N'-[1,1-bis(oxidanylidene)thian-4-yl]-5-ethyl-4-oxidanylidene-7-[3-(trifluoromethyl)phenyl]thieno[3,2-c]pyridine-2-carboximidamide 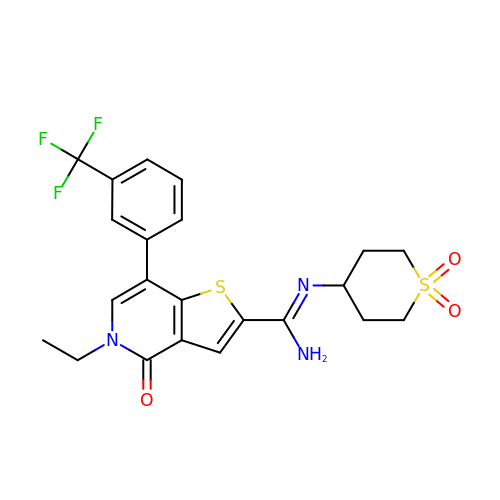| C22 H22 F3 N3 O3 S2 | WRUWGLUCNBMGPS-UHFFFAOYSA-N> GHMQETQAVEAGEKTVEQFVQALNKGDYNKAAEMTSKKAANKSALSEKEILDKYQNIYGAADVKGLQISNLKVDKKDDSTYSFSYKAKMNTSLGELKDLSYKGTLDRNDGQTTINWQPNLVFPEMEGNDKVSLTTQEAARGNIIDRNGEPLATTGKLKQLGVVPSKLGDGGEKTANIKAIASSFDLTEDAINQAISQSWVQPDYFVPLKIIDGATPELPAGATIQEVDGRYYPLGEAAAQLIGYVGDITAEDIDKNPELSSNGKIGRSGLEMAFDKDLRGTTGGKLSITDADGVEKKVLIEHEVQNGKDIKLTIDAKAQKTAFDSLGGKAGSTVATTPKTGDLLALASSPSYDPNKMTNGISQEDYKAYEENPEQPFISRFATGYAPGSTFKMITAAIGLDNGTIDPNEVLTINGLKWQKDSSWGSYQVTRVSDVSQVDLKTALIYSDNIYMAQETLKMGEKK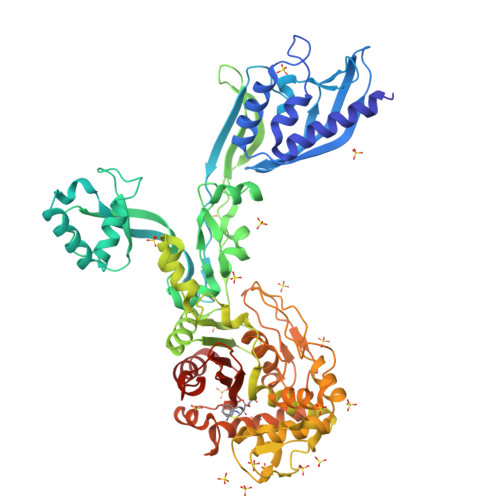FRIGLDKFIFGEDLDLPISMNPAQISNEDSFNSDILLADTGYGQGELLINPIQQAAMYSVFANNGTLVYPKLIADKETKDKKNVIGETAVQTIVPDLREVVQDVNGTAHSLSALGIPLAAKTGTAEIKEKQDEKGKENSFLFAFNPDNQGYMMVSMLENKEDDDSATKRASELLQYLNQNYQ> MASMKVAVLPGDGIGPEVTEAALKVLRALDEAEGLGLAYEVFPFGGAAIDAFGEPFPEPTRKGVEEAEAVLLGSVGGPKWDGLPRKIRPETGLLSLRKSQDLFANLRPAKVFPGLERLSPLKEEIARGVDVLIVRELTGGIYF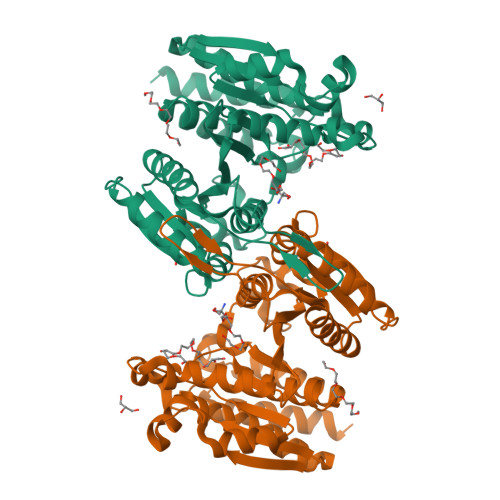GEPRGMSEAEAWNTERYSKPEVERVARVAFEAARKRRKHVVSVDKANVLEVGEFWRKTVEEVGRGYPDVALEHQYVDAMAMHLVRSPARFDVVVTGNIFGDILSDLASVLPGSLGLLPSASLGRGTPVFEPVHGSAPDIAGKGIANPTAAILSAAMMLEHAFGLVELARKVEDAVAKALLETPPPDLGGSAGTEAFTATVLRHLAAAALEHHHHHH>DISPDGAQSCSPIQLYAIPPSPGELYISLDAKLRCLVVNLPSDSSLSVTWTREKSGNLRPDPMVLQEHFNGTYSASSAVPVSTQDWLSGERFTCTVQHEELPLPLSKSVYRNTGPTTPPLIYPFAPHPEELSLSRVTLSCLVRGFRPRDIEIRWLRDHRAVPATEFVTTAVLPEERTANGAGGDGDTFFVYSKMSVETAKWNGGTVF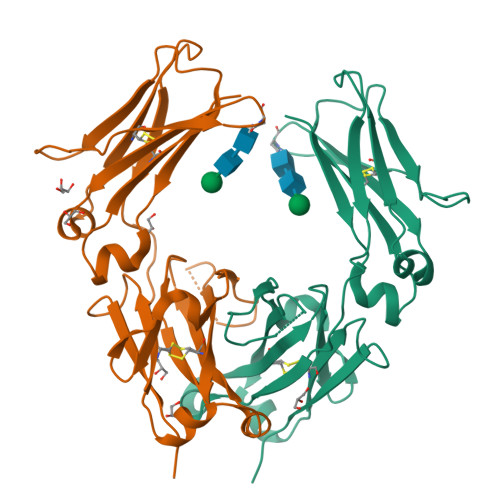ACMAVHEALPMRFSQRTLQKQAGK[2x]> GCGTGCCGCATTA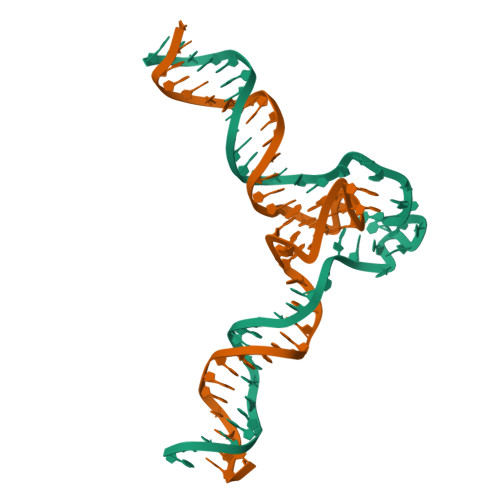ATTTTTTTTTTTTTTTTTTTTTTGTATACATAG;> CTATGTATACAAAGAGGGTGGGTAGGGTGGGTTTAATGCGGCACGC> MFADTAALKAAMDTALKEHPDKPVVLDFYADWCISCKEMAAYTLNQPEVHQAVDMERFFQIDVTANKPEHQALLKEYGLFGPPGVFV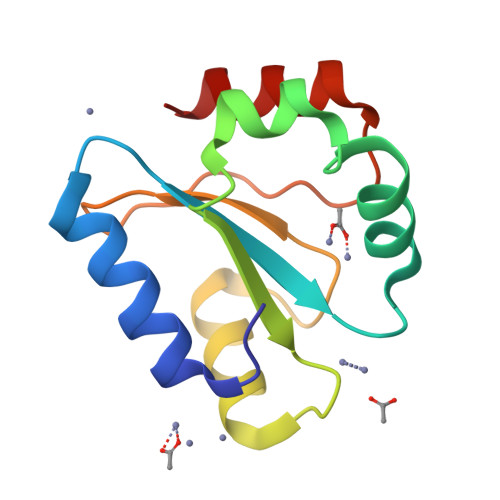VRSDGSRSEPLLGFVKADKFIEWYEQNR> HHHHHHHHHHSSGHIEGRHMAGLRHTFVVADATLPDCPLVYASEGFYAMTGYGPDEVLGHNCRFLQGEGTDPKEVQKIRDAIKKGEACSVRLLNYRKDGTPFWNLLTVTPIKTPDGRVSKFVGVQVDVTSKTEGKALA

Light–oxygen–voltage (LOV) domains are small photosensory flavoprotein modules that allow the conversion of external stimuli (sunlight) into intra­cellular signals responsible for various cell behaviors (e.g. phototropism and chloro­plast relocation). This ability relies on the light-induced formation of a covalent thio­ether adduct between a flavin chromophore and a reactive cysteine from the protein environment, which triggers a cascade of structural changes that result in the activation of a serine/threonine (Ser/Thr) kinase. For example, in the green algae Chlamydomonas reinhardtii (C. reinhardtii or Cr), phot allows the light-dependent regulation of several molecular processes (e.g. phototaxis, sexual differentiation, photoprotection) and control of gene expression. The C. reinhardtii phot protein consists of two successive photosensory protein modules, LOV1 and LOV2 domains, and a Ser/Thr kinase effector domain [Fig. 1(a)].

As expected from the CT characterization, the CrPhot­LOV1 crystals belonged to the P6522 space group. We used the model coordinates of the CT dark-state structure to calculate initial phases and then manually adjusted them with Coot before refining them with Phenix. Overall, the electron density was of excellent quality and enabled us to observe variations in the positions of residue side chains (with an RMSD of 0.189 Å between the dark state at CT and RT). The reactive cysteine (Cys57) exhibited two alternate conformations, as observed at CT, but the variation of the 2Fo − Fc map contour at RT clearly indicated a change in the distribution of each conformation [Figs. 3(a) and 3(b), respectively]. Conformation A, in which the Sγ atom of Cys57 is 3.5 Å from the C4a of FMN, was equally present at RT along with conformation B (i.e. 0.50 and 0.50 for A and B conformations, respectively), in which the Sγ atom of Cys57 is 4.4 Å from the C4a of FMN.>NVGSNTY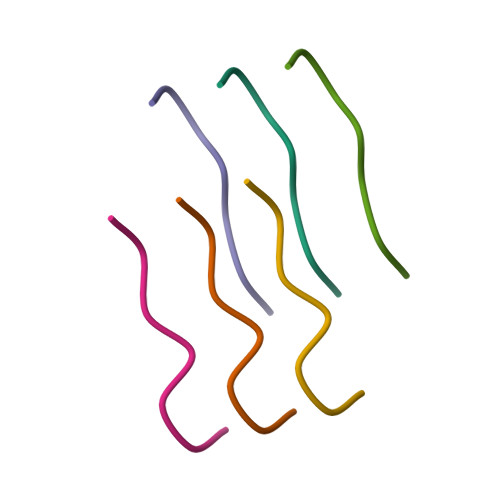[2x]>[8x]MAETLIKVDLNQSPYDNPQVHNRWHPDIPMAVWVEPGAEFKLETYDWTGGAIKNDDSAEDVRDVDLSTVHFLSGPVGVKGAEPGDLLVVDLLDIGARDDSLWGFNGFFSKQNGGGFLDEHFPLAQKSIWDFHGMFTKSRHIPGVNFAGLIHPGLIGCLPDPKMLASWNERETGLIATDPDRIPGLANPPNATTAHMGQMQGEARDKAAAEGARTVPPREHGGNCDIKDLSRGSRVFFPVYVDGA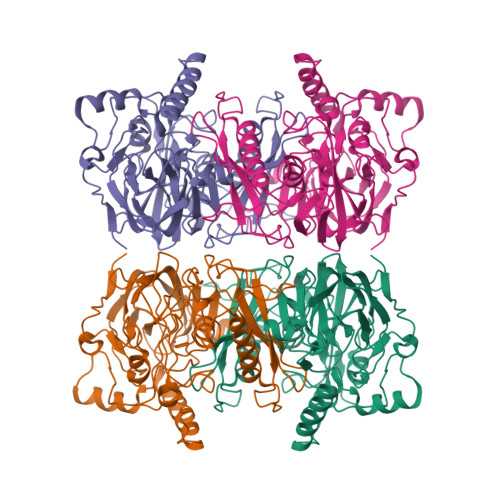GLSVGDLHFSQGDGEITFCGAIEMAGWVHMKVSLIKGGMAKYGIKNPIFKPSPMTPNYKDYLIFEGISVDEKGKQHYLDVTVAYRQACLNAIEYLKKFGYSGAQAYSLLGTAPVQGHISGVVDVPNACATLWLPTEIFDFDINPTAEGPQKIITGGVDLPIAQDK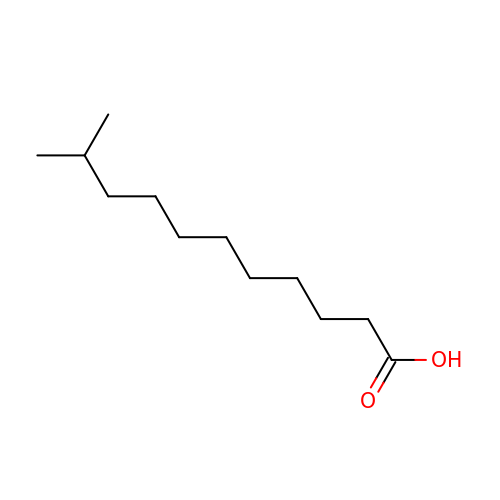10-METHYLUNDECANOIC ACID | C12 H24 O2 | QJRRBVNPIKYRQJ-UHFFFAOYSA-N>MSDTVEWFKQAKYGMMIHWGLYSLLGGEYQGKSSSNYAEWVQSKLQIPNKEYERLTQAFNPIYFDADAIIDLAKRCGMQYLVVTTKHHDGFAMYRSLVDPYNVYDATPFHRDVIGELSLACRKAGLRFGLYYSQDLDWHEPDGGGYLSNDIETAGTTWDNSWDFTGEKNYDRAFKHKIMPQIEEIMSNYGEISVAWFDVPMTLSDEQSQTIYDTVKRLQPDCLINSRLGNGRYDYVSLGDNEIPEDSDASDKATSDGNVDYNSIEGFKPSKLGLYETAGTINDSWGFAYHDQNWKSPQTIHDYKAHLNKYGINYLLNVGLDGLGRVPMAAEQALLGARALEA[6x]

Microbial α-l-fucosidases catalyse the hydrolysis of terminal α-l-fucosidic linkages and can perform transglycosylation reactions. In contrast, fucosidases from the GH29 family have been widely studied since 1970s9 and are reported to act on a broad range of substrates with hydrolysis proceeding via a retaining mechanism. The structural basis for the substrate specificity of GH29 fucosidase from Bifidobacterium asteroides towards α1,6 linkages and FA2G2 N-glycan was determined by X-ray crystallography and STD NMR. Here, we showed that BaGH2926A from B. asteroides, in cluster 26, exhibited α1,6 substrate specificity and could hydrolyse FA2G2 N-glycan through recognition of 6FN epitopes, as shown by STD NMR but could not release Fuc from N-glycan unlike GH29-BifC, indicating that GH29-BifC and GH29-BifD differ in their capacity to accommodate the reducing end of N-glycan.

X-ray crystallography was used to gain structural insights into BaGH2926A α1,6 specificity. It was only possible to grow diffracting crystals of BaGH2926A wild-type (WT) in the presence of 2’FL, resulting in a complex with Fuc bound in the active site while the nucleophile mutant BaGH2926AD128N was crystallised in an apo-form (Supplementary Data 1&2). BaGH2926A WT and mutant displayed a (α/β)8-fold, typical of GH29 enzymes. Asp218 was identified as the catalytic nucleophile based on its homology with other GH29 enzymes and proximity to the Fuc residue (2.9 Å from the ring oxygen of the bound sugar). We propose Asp260 as the putative acid/base residue based on its superimposition with Asp242 of AlfC26A from Lactobacillus casei W56, although this catalytic residue was not experimentally validated. Extensive hydrogen bonding interactions were observed between the active site and the bound sugar hydroxyl groups. The C6 methyl group sits in a hydrophobic pocket formed by Trp216 and Trp305. Unlike E1_101251B, which showed evidence of β-fucose bound, the electron density of the BaGH2926A complex most clearly matched α-Fuc. Compared to fucosidases E1_101251B from R. gnavus E1 and Blon_23361B from B. longum subsp. infantis, the BaGH2926A active site was shown to be constricted, which may contribute to the substrate specificity of this enzyme. Tyr57 may be implicated in BaGH2926A α1,6 linkage specificity. From closer inspection of the active site, it is expected that BaGH2926A Ile284 would clash with substrates presenting α1,3/4 linkages, whereas the presence of an acidic residue in this position in Blon_23361B would create a stabilising hydrogen bond to the substrate.> ERYENLFAQLNDRREGAFVPFVTLGDPGIEQSLKIIDTLIDAGADALELGVPFSDPLADGPTIQNANLRAFAAGVTPAQCFEMLALIREKHPTIPIGLLMYANLVFNNGIDAFYARCEQVGVDSVLVADVPVEESAPFRQAALRHNIAPIFICPPNADDDLLRQVASYGRGYTYLLSRSGVTGAENRGALPLHHLIEKLKEYHAAPALQGFGISSPEQVSAAVR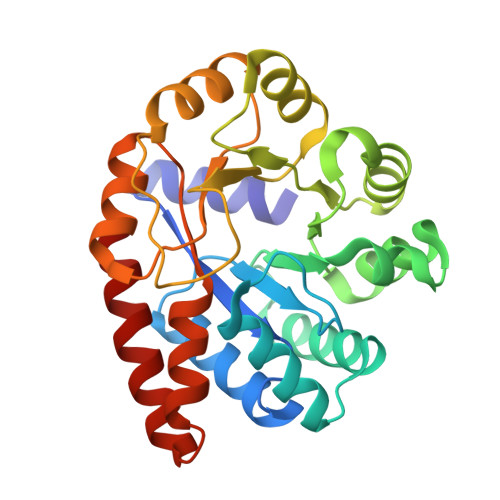AGAAGAISGSAIVKIIEKNLASPKQMLAELRSFVSAMKAASR>[12x]MLVFIDDGSTNIKLQWQESDGTIKQHISPNSFKREWAVSFGDKKVFNYTLNGEQYSFDPISPD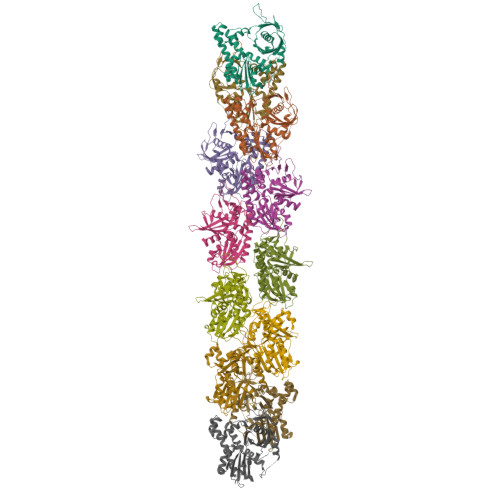AVVTTNIAWQYSDVNVVAVHHALLTSGLPVSEVDIVCTLPLTEYYDRNNQPNTENIERKKANFRKKITLNGGDTFTIKDVKVMPESIPAGYEVLQELDELDSLLIIDLGGTTLDISQVMGKLSGISKIYGDSSLGVSLVTSAVKDALSLARTKGSSYLADDIIIHRKDNNYLKQRINDENKISIVTEAMNEALRKLEQRVLNTLNEFSGYTHVMVIGGGAELICDAVKKHTQIRDERFFKTNNSQYDLVNGMYLIGN>[2x]MKPPFQEALGIIQQLKQHGYDAYFVGGAVRDLLLGRPIGDVDIATSALPEDVMAIFPKTIDVGSKHGTVVVVHKGKAYEVTTFKTDGDYEDYRRPESVTFVRSLEEDLKRRDFTMNAIAMDEYGTIIDPFGGREAIRRRIIRTVGEAEKRFREDALRMMRAVRFVSELGFALAPDTEQAIVQNAPLLAHISVERMTMEMEKLLGGPFAARA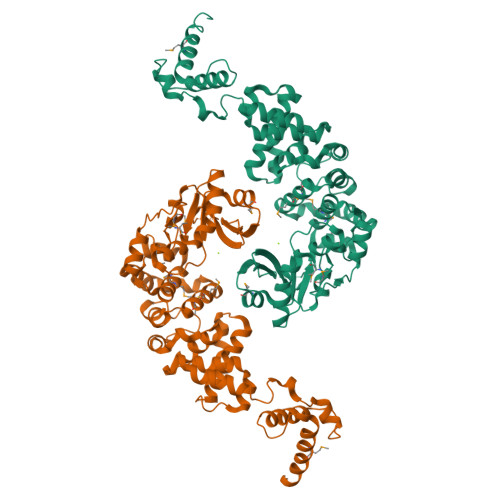LPLLAETGLNAYLPGLAGKEKQLRLAAAYRWPWLAAREERWALLCHALGVQESRPFLRAWKLPNKVVDEAGAILTALADIPRPEAWTNEQLFSAGLERALSVETVRAAFTGAPPGPWHEKLRRRFASLPIKTKGELAVNGKDVIEWVGKPAGPWVKEALDAIWRAVVNGEVENEKERIYAWLMERNRTREKNC>[2x]MAKKTSSKGKLPPGPRPLPLLGNLLQMDRRGLLKSFLRFREKYGDVFTVHLGPRPVVMLCGVEAIREALVDKAEAFSGRGKIAMVDPFFRGYGVIFANGNRWKVLRRFSVTTMRDFGMGKRSVEERIQEEAQCLIEELRKSKGALMDPTFLFQSITANI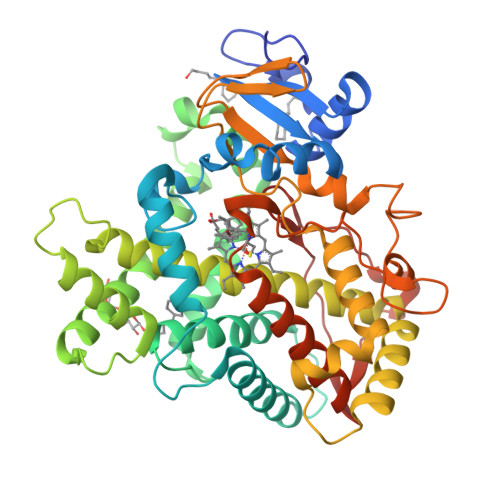ICSIVFGKRFHYQDQEFLKMLNLFYQTFSLISSVFGQLFELFSGFLKHFPGAHRQVYKNLQEINAYIGHSVEKHRETLDPSAPRDLIDTYLLHMEKEKSNAHSEFSHQNLNLNTLSLFFAGTETTSTTLRYGFLLMLKYPHVAERVYREIEQVIGPHRPPELHDRAKMPYTEAVIYEIQRFSDLLPMGVPHIVTQHTSFRGYIIPKDTEVFLILSTALHDPHYFEKPDAFNPDHFLDANGALKKTEAFIPFSLGKRICLGEGIARAELFLFFTTILQNFSMASPVAPEDIDLTPQECGVGKIPPTYQIRFLPRHHHH>[22x]TGTANTLFGTAS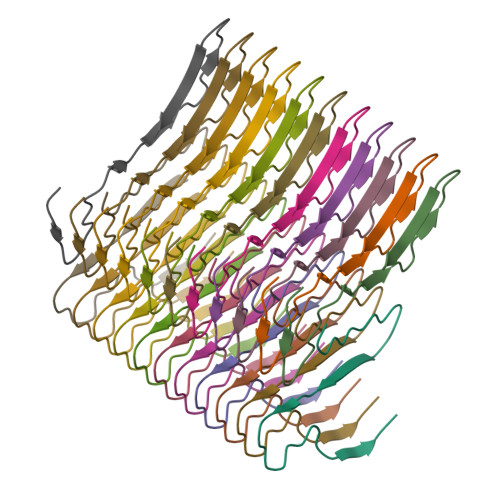TGTSLFSSQNNAFAQNKPTGFGNFGTST> DCPPDWSSYEGHCYRFFKEWMHWDDAEEFCTEQQTGAHLVSFQSKEEADFVRSLTSEMLKGDVVWIGL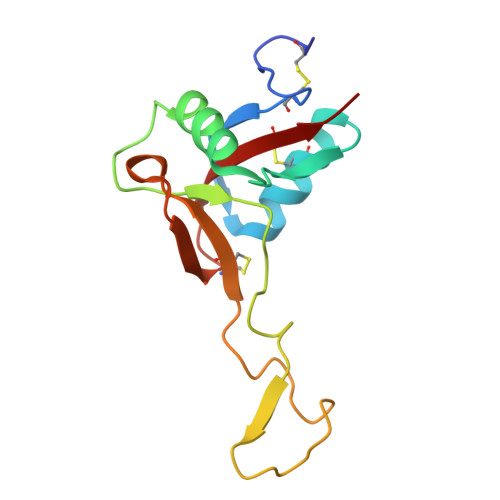SDVWNKCRFEWTDGMEFDYDDYYLIAEYECVASKPTNNKWWIIPCTRFKNFVCEFQA> MHHHHHHLEGSDLEICSLPKSLFQEQWSQFKLTHKKSYSSPIEEIRRQLIFKDNVAKIAEHNAKFEKGEVTYSKAMNQFGDMSKEEFLAYVNRGKAQKPKHPENLRMPYVSSKKPL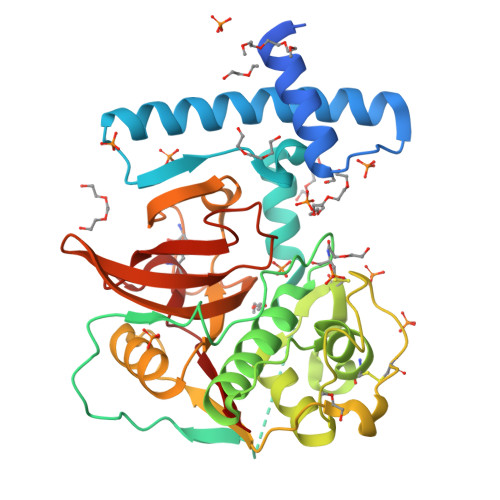AASVDWRSNAVSEVKDQGQCGSSWSFSTTGAVEGQLALQRGRLTSLSEQNLIDCSSSYGNAGCDGGWMDSAFSYIHDYGIMSESAYPYEAQGDYCRFDSSQSVTTLSGYYDLPSGDENSLADAVGQAGPVAVAIDATDELQFYSGGLFYDQTCNQSDLNHGVLVVGYGSDNGQDYWILKNSWGSGWGESGYWRQVRNYGNNCGIATAASYPAL> MAEEHHHHHHHHLEVLFQGPPPGPRSPQREPQRVSHEQFRAALQLVVDPGDPRSYLDNFIKIGEGSTGIVCIATVRSSGKLVAVKKMDLRKQQRRELLFNEVVIMRDYQHENVVEMYNSYLVGDELWVVMEFLEGGALTDIVTHTRMNEEQIAAVCLAVLQALSVLHAQGVIHRDIKSDSILLTHDGRVKLSDFGFCAQVSKEVPRRKSLVGTPYWMAPELISRLPYGPEVDIWSLGIMVIEMVDGEPPYFNEPPLKAMKMIRDNLPPRLKNLHKVSPSLKGFLDRLLVRDPAQRATAAELLKHPFLAKAGPPASIVPLMRQNRTR;> AEDWTAALLN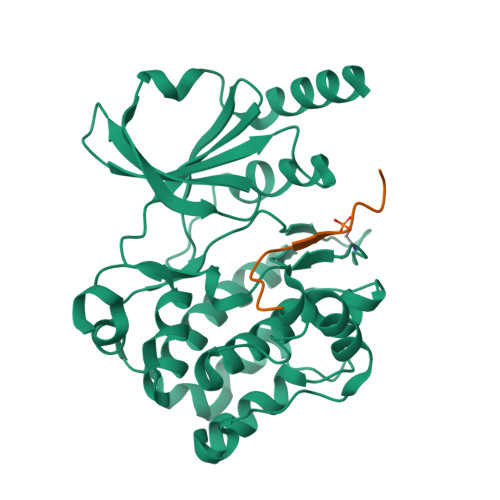RGRSRQPLVLGDNC>[2x]MTTLFDP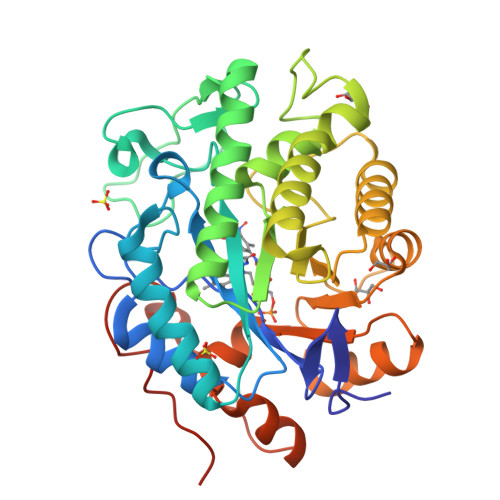IKLGDLQLPNRIIMAPLTRCRADEGRVPNALMAEYYVQRASAGLILSEATSVSPMGVGYPDTPGIWNDEQVRGWNNVTKAVHAAGGRIFLQLWHVGRISHPSYLNGELPVAPSAIQPKGHVSLVRPLSDYPTPRALETEEINDIVEAYRSGAENAKAAGFDGVEIHGANGYLLDQFLQSSTNQRTDRYGGSLENRARLLLEVTDAAIEVWGAQRVGVHLAPRADAHDMGDADRAETFTYVARELGKRGIAFICSREREADDSIGPLIKEAFGGPYIVNERFDKASANAALASGKADAVAFGVPFIANPDLPARLAADAPLNEAHPETFYGKGPVGYIDYPRLKLAAALEHHHHHH> MQTKERYQLQRLTLLALLTAMCVVLRIFKIIDIPNVQPVTDIIMLTTLELGAGTGILLAILVMVISNIFLGFGIWTLPQIF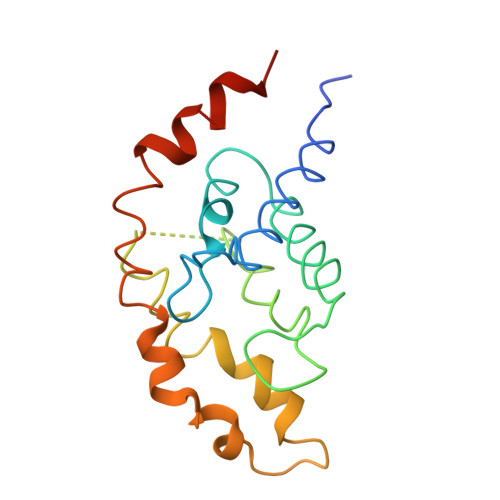AYAACALTVALFARLLPLKSRKFFWLQELLAGFLGLEYGFFVSLGMAGWGGWAAFIAYWVSGLTFDLYHAAGNLAFYPIFYLPLVLGLDRFKKKAGWKQNA>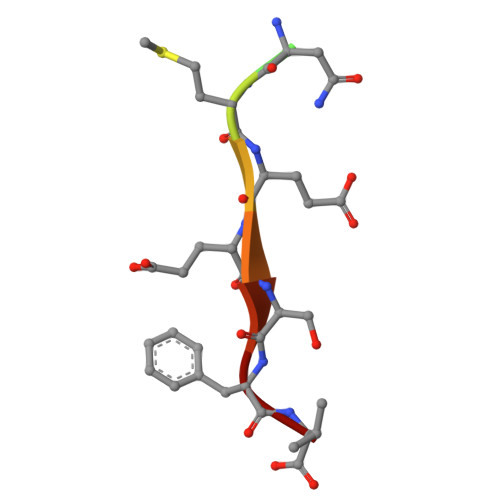 LCSNMEESFV> GPGSMSNVAVNTVF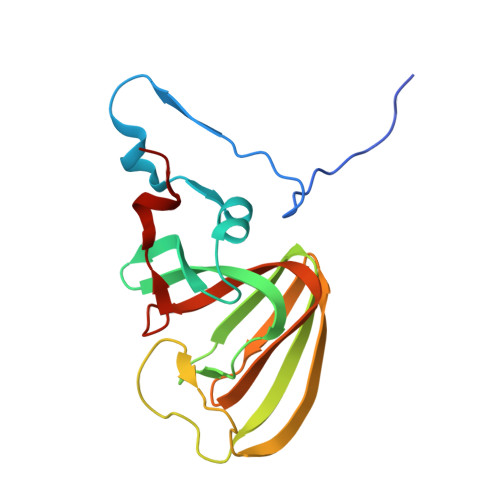ASLDNFRKGTVEIISGEARHYAFSNIFEVAQNSKPYEKVVVGLNLGYVVETLRAEGQSPWFTAAHDEFAIVMDGEVRVEFLKLDAPSKHGEGTHLAGELPVGKPMGYVLLKRGHQCLLPAGSAYRFEASRPGVILQQTIKGPLSVEKWAEICLK>[2x]MDTNPCEKHSCIAVIDAGSTGSRLHIYSYDTDDTNTPIHIEEIWNKKIKPGFASIQPNSVTIDAYLTMLLADAPIHNIPVYFYATAGMRLLPQSQQKKYYDELDYWFRQQSQWQLVEAKTITGNDEALFD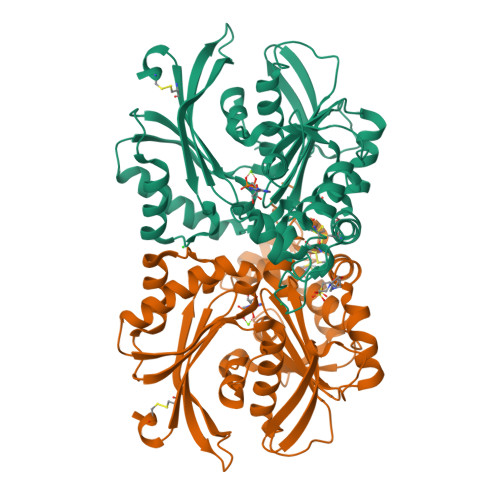WLAVNYKLDTLKSVQNKSVGVMDMGGASVQIVFPMPKNAEISKHNQVELNIYGQNINLYVHSFLGLGQTEMSHQFLNSPSCFANDYPLPDGESGQGNAPSCKEEVTSLMNSVHKVNQQIQPLLALNPVNEWYSIGGISNLASSQLFHFENSELTNQSLLQQGDNQICHQQWDILNGQYPDDEYLYQYCLLSSYYYALMVDGYGINPNQTIHYIPPEQNLDWTIGVVLHRALEHHHHHH> MTGKKTLSIVGASGYAGGEFLRLALSHPYLEVKQVTSRRFAGE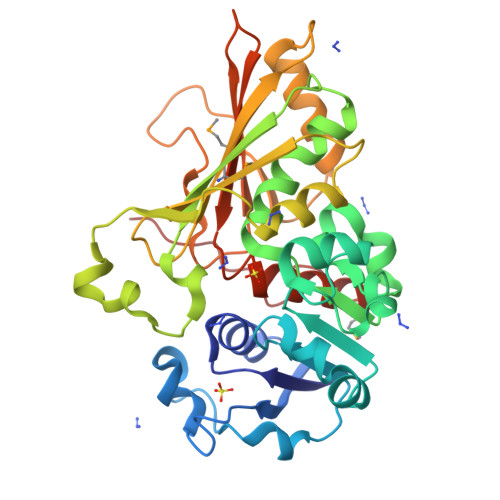PVHFVHPNLRGRTNLKFVPPEKLEPADILVLALPHGVFAREFDRYSALAPVLVDLSADFRLKDPELYRRYYGEHPRPDLLGRFVYAVPELYREALKGADWIAGAGCNATATLLGLYPLLKAGVLKPTPIFVTLLISTSAGGAEASPASHHPERAGSIRVYKPTGHRHTAEVVENLPGRPEVHLTAIATDRVRGILMTAQCFVQDGWSERDVWQAYREAYAGEPFIRLVKQKKGVHRYPDPRFVQGTNYADIGFELEEDTGRLVVMTAIDNLVKGTAGHALQALNVRMGWPETLGLDFPGLHP> ST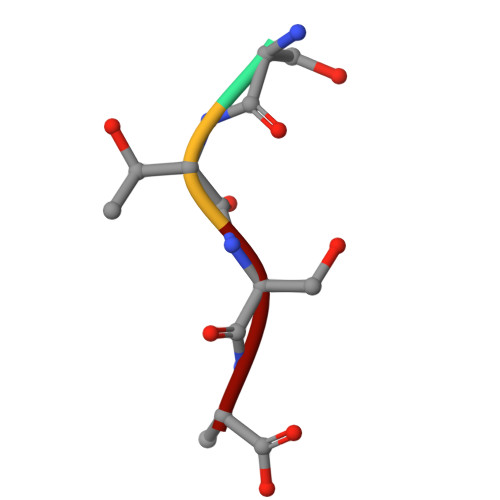SA>MSENKATLMEGMTEKTLHSPNTMAEVASLHVANSYIGTGLDTSLENVKPLPEACKRNVTEFDLVAYGKDEFTLSMEKRVMARMFSAFDVTQLGYLEERKIEHMCKYLGRVMNEDDVKQMKSEINAIDGHITFEKFWAWWCSHPEVPAKKDFFSMVSVDFAVPYHQQQLLTRETGELYTPSYRVLYYFRDMETGKELQVSPWHDIPLYVRDLVRTKPASLPMNRYNFICEIPKWTRAKFEIATGEPFNPIKQDIKNGVPRFYKHGDMMWNYGALPQTWESTDVVFEGGYVGDNDPIDAIEIGMTQFKVGQVGAVKVLGILGMIDDGQMDWKVICISHNDPICRFLKDIHDVPKFLPGCLDAIHEWFRVYKICQGGVENKFVFNGEFKDKSFAMKVIDESHYMWGNLRKI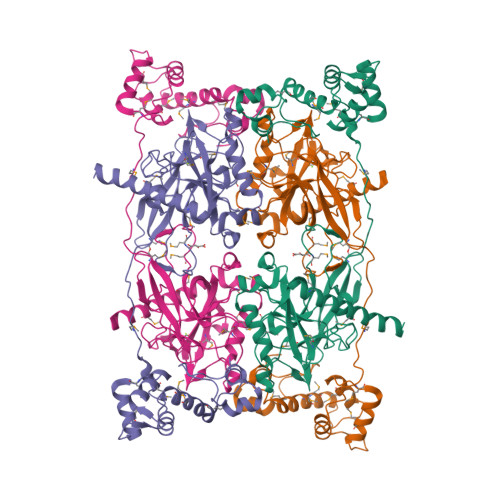NKKEEV[2x]>MSKWTYFGPDGENSWSKKYPSCGGLLQSPIDLHSDILQYDASLTPLEFQGYNLSANKQFLLTNNGHSVKLNLPSDMHIQGLQSRYSATQLHLHWGNPNDPHGSEHTVSGQHFAAELHIVHYNSDLYPDASTASNKSEGLAVLAVLIEMGSFNPSYDKIFSHLQHVKYKGQEAFVPGFNIEELLPERTAEYYRYRGSLTTPPCNPTVLWTVFRNPVQISQEQLLALETALYCTHMDDPSPREMINNFRQVQKFDERLVYTSFSQ[2x]

The role of carbonic anhydrase isozyme IX (CAIX) in tumor cell survival, proliferation, migration, pH regulation, and cell-signaling pathways made this enzyme a promising therapeutic target in oncology. , Tumor cells primarily express two membrane-associated carbonic anhydrases, CAIX and CAXII. These isozymes belong to a family of zinc metalloenzymes that catalyze the reversible hydration of CO2 to form HCO3 – and H+. Although the active site is characterized by conserved amino acids between 12 isozymes, the amino acids further away from the zinc ion provide some variability. Crystal structures of CAIX and CAXII with five compounds by using soaking or cocrystallization were determined to confirm the binding mode of the ligands and reveal insights that govern enhanced affinity.

Four ligands in complexes with CAXII are of similar structures, contain a cyclooctylamine group at the 3-position and (3-hydroxypropyl)­sulfonyl tail at the 4-position, but vary in substituents at the 5-position: compound 9 has a (4-hydroxybutyl)­amino moiety, compound 10 - piperidinyl, compound 13 - methoxy, and compound 14 - ethoxy. Compound 10 with cyclic piperidinyl group retains a high affinity for CAIX (K d,obs 0.29 nM). A complex of CAXII-10 is present in structures containing two and four subunits. In all subunits, the ligand adopts a consistent binding mode, with variability in the cyclooctylamino and piperidinyl rings. Additionally, the para-tail hydroxyl group shows positional variability, as it is exposed to solvent. The meta-piperidinyl group in compound 10 is well-stabilized and tightly packed against the hydrophilic cavity wall, with all conformations being similar. Like compound 13, a water molecule is also found in a similar position and forms hydrogen bonds with Y6 and H67. However, there is no direct interaction between this meta-substituent of the ligand and the protein. The sulfoxide linker of the para-tail is stabilized by a hydrogen bond with N64 and Q89, except in CAXII-10, where N64 is too distant for interaction, but in one subunit 3.4 Å hydrogen bond is still possible. Interestingly, despite the bulkiness of synthesized di-meta-substituted compounds 10, 13, and 14, especially the first one compound 10, which possesses large piperidinyl and cyclooctylamino groups, ligands acquire quite similar binding poses in the soaked and cocrystallized complexes with CAXII.> GHFKDPKRLY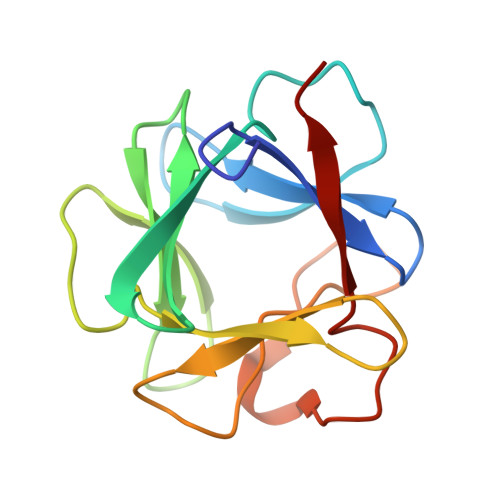CKNGGFFLRIHPDGRVDGVREKSDPHIKLQLQAEERGVVSIKGVSANRYLAMKEDGRLLASKSVTDECFFFERLESNNYNTYRSRKYTSWYVALKRTGQYKLGSKTGPGQKAILFLPMSAKS> SFEGY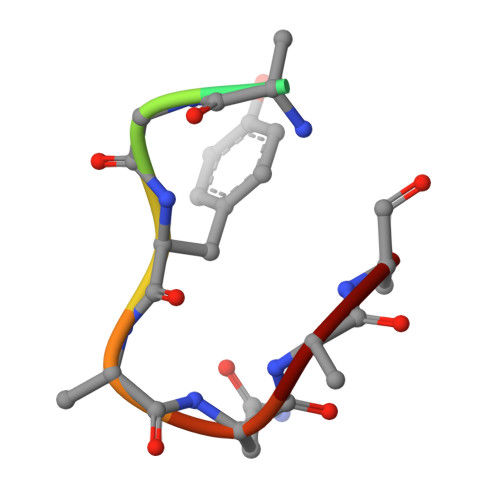DNSC>MAHHHHHHKIEENQNVSLNEGDIVSKLKETPQETLVPTKWDVGDTTVSNEDRLDLLIPHVQNLGNVYVGVGSEQNLTIAAWAKSDFIYLMDFTQIVVHANTITILFLQKSEKKEDFIRLWGKEGEKEALELIQVSFSDPEVYKKVYKQASPFIRKRHKTNLMLSKKYNYKMFQTDDEQYSYIRKLAIEGKILPIRGNLLGNITLTGIGNTLKKIGRKVGIIYFSNAEEYFAYPQEFKNSILNLPVSESSLVVRTISVRKDLFPWSPGSEISTDRGFHYCVQKISNFQKWLSSGKPGLRSLQVMVEGGTVDKKNGITVVDKE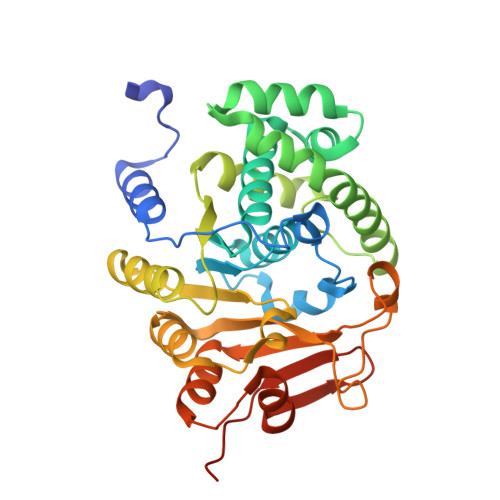PVVTEDKLPKTGG[2x]>GSHMAVELNH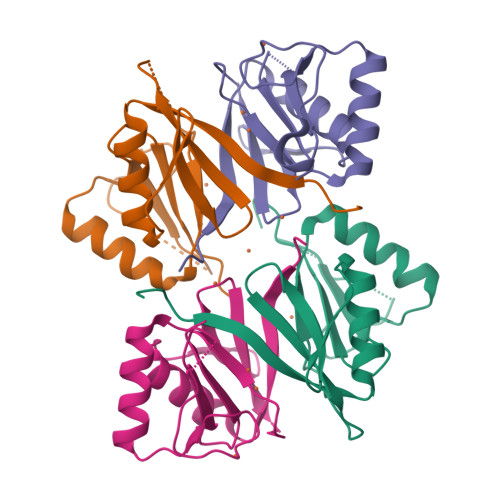TIVLVKDKDASATFMADLLGLPKPKEMGPFAVLQLANDVSILFMDFRGEGDIVPGHCAFLISDEEFDQIFGRIREGGIEHWADQYHREPGRINDRDGGRGVYFEDPSGHNMEIMTRPYGSGGA[4x]>[2x]MAHHHHHHESETTTSLVLERSLNRVHLLGRVGQDPVLRQVEGKNPVTIFSLATNEMWRSGDSEVYQLGDVSQKTTWHRI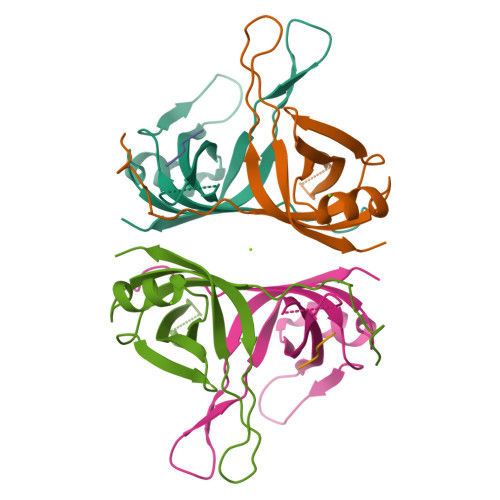SVFRPGLRDVAYQYVKKGSRIYLEGKIDYGEYMDKNNVRRQATTIIADNIIFLSDQTKEKELE;> SSSS>MVNVEEIRKAQRAEGPAAILAIGTATPPNAIEQSEYPDYYFRVTNSEDKVELKEKFKRMCEKSMIKKRYLYLTEDILKENPNVCAYMATSLDARQDMVVVEVPKLGKEAATRAIKEWGQPKSKITHLVFCTTSGVDMPGADYQLTKLLGLRPSVKRLMMYQQGCFAGGTVLRLAKDLAENNRGARVLVVCSEITAVTFRGPSESHLDSLVGQALFGDGAAALIVGSDAIEGIERPIFEMVSAAQTILPDSEGAIDGHLREVGLTFHLLKDVPGIISKNIEKSLEEAFKPLGITDYNSLFWIAHPGGPAILDQVEAKIGLKPEKLRATRHVLSEYGNMSSACVLFIL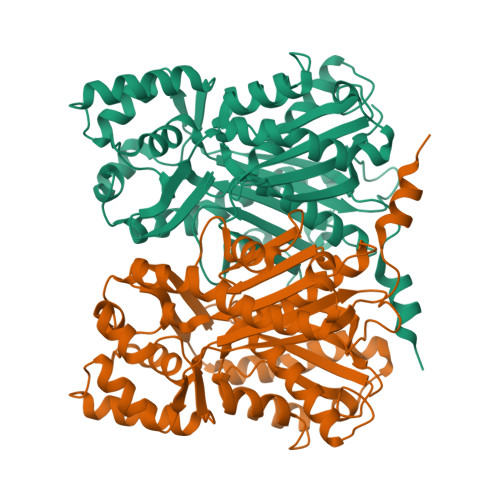EEMRKKSAEEKNGTTGEGLEWGVLFGFGPGLTVETVVLHSVEA[4x]> MKKNKKTTKSLLSADEKITESLRSTLSDVLPDQLQTYIRTVLQFSGRPEGANLLTGPNTEIEFFSQDPNKNFPNIFAKYSNVLTVSSDPNFITSEDEEVKIIWGRHGSDSLIGFDPGADLVGKRRIDIFLGDFIDEQFNPIPGALNAGKSWSDRFILGDWQKPYYFEDDETLGLNQSAMILDFNPNEDVIQLHGDRQDYELVNISLGTAIFWREKKGYDLIGVLGGVSDLSLKGDYFEFKGNTAPKTVLKTAEHIGTAANDYIFSSTVDAKGNFYVGGGTGGSLGGRNIGARDAWLAKYDSNGNQRWSRQFGSTGTESLWGMASDGSNIYVAGNTTGQLENNTVKGGNDAYLAKYDSDGNQVWIKQNGTYTLEESYKITVDSSGNIYTAGHTFGSLGGPNQNLEQGEVFELPSTDGYVAKFDSNGNQLWVAQFGTITLDDNWGVAADNNGNVFAGGNTKGSFGAKNTGTAGEYDAWLVKLNKDGQTDWV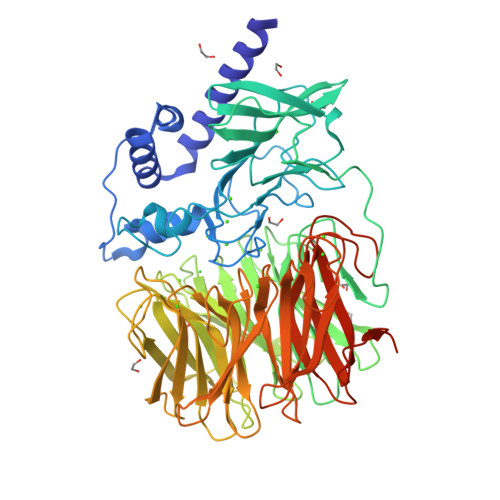RQFGTPNYDFMWDIETDSLGDIYATGWTLGDLGGKNAGSYDVWLAKYNTNGNQLWIKQFGTSEDDAPFLDGIDIDANDNIFLTGNTNGNLGGANAGSYDAWAAKFDKDGNQLWLKQFGTPDYDTATTVTAVNFGKLYVSGITEGSLGTTNAGSYDSWALKLDADNGEIQDFNSSTNTFGQTGFLNLGSAWSHPQFEK> SMQLNQYTLKDEIGKGSYGVVKLAYNENDNTYYAMKVLSKKKLIRQAGFPRRPPPRGTRPAPGGCIQPRGPIEQVYQEIAILKKLDHPNVVKLVEVLDDPNEDHLYMVFELVNQGPVMEVPTLKPLSEDQARFYFQDLIKGIEYLHYQKIIHRDIKPSNLLVGEDGHIKIADFGVSNEFKGSDALLSNTVGTPAFMAPESLSETRKIFSGKALDVWAMGVTLYCFVFGQCPFMDERIMCLHSKIKSQALEFPDQPDIAEDLKDLITRMLDKNPESRIVVPEIKLHPWVTRH

Protein kinases catalyze phosphate transfer from Adenosine Triphosphate (ATP) to tyrosine, threonine or serine residues in specific target proteins. CaMKK2 is predominantly expressed in the brain, with trace expression in peripheral tissues such as the testis, spleen and lung. In addition to recently being linked to appetite in vivo, CAMKK2 is over-expressed in multiple cancers. The knockout of CaMKK2 can reduce cell proliferation and tumorigenicity in vivo, making CAMKK2 an attractive drug target.

Diffracting crystals were obtained with compound 2 in complex with CAMKK2. The CAMKK2 kinase domain adopted an active state conformation in which residues of the regulatory and catalytic spines were aligned; residue Glu236 within α-C helix directly contacted Lys194 (“α-C helix in”); and residues Asp330 and Phe331 within the conserved DFG motif pointed towards and away, respectively, from the ATP-binding site (“DFG -in”). The ligand displayed two direct contact points to the hinge region of the ATP-binding pocket: one involving the oxygen atom of the thiadiazinone moiety and the other through the nitrogen atom of the hydroxymethylaniline moiety. A water bridge made by the nitrogen atom from the aminobenzamide provided a third contact point to the kinase hinge region. The co-crystal structure revealed that the oxygen atom of the aminobenzamide interacted with the catalytic Lys194 and made a water-bridge with Glu236 of the α-C helix and Asp330 within the conserved DFG motif. Likewise, two water-bridge interactions connected the nitrogen atom from the aminobenzamide moiety and residues Ser175 within P-loop and Asn317 at the bottom of the kinase ATP-binding site. Finally, the ligand aminobenzamide ring made a T-shaped π-π interaction with the Phe267. Compound 2 is bound to CAMKK2 with aniline groups in a twisted conformation relative to the central TDZ ring, as can be seen in the electron density map. We noted that STO-609 can displace a bound water molecule from the ATP-binding site that is still present when compound 2 is bound to the enzyme. We demonstrate, for the first time, that the 4H-1,2,6-thiadiazin-4-one (TDZ) chemotype can function as an ATP-competitive kinase inhibitor.~{N}-[(2~{R},3~{R},4~{R},5~{S},6~{R})-6-(hydroxymethyl)-5-[(2~{S},3~{R},4~{S},5~{S},6~{R})-6-(hydroxymethyl)-4-[(1-methyl-1,2,3-triazol-4-yl)methoxy]-3,5-bis(oxidanyl)oxan-2-yl]oxy-4-oxidanyl-2-propoxy-oxan-3-yl]ethanamide 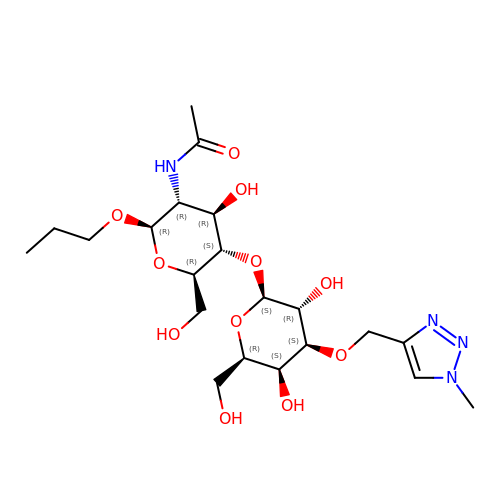| C21 H36 N4 O11 | MSOLTVRMDPXMPE-WFNKYQNYSA-N>MALEEIRPKEVYLD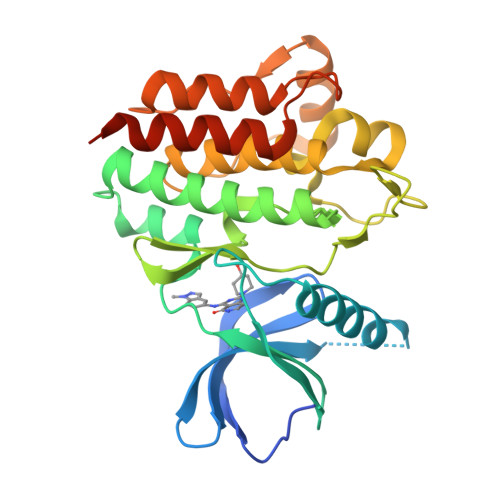RKLLTLEDKELGSGNFGTVKKGYYQMKKVVKTVAVKILKNEANDPALKDELLAEANVMQQLDNPYIVRMIGICEAESWMLVMEMAELGPLNKYLQQNRHVKDKNIIELVHQVSMGMKYLEESNFVHRDLAARNVLLVTQHYAKISDFGLSKALRADENYYKAQTHGKWPVKWYAPECINYYKFSSKSDVWSFGVLMWEAFSYGQKPYRGMKGSEVTAMLEKGERMGCPAGCPREMYDLMNLCWTYDVENRPGFAAVELRLRNYYYDVVNLEHHHHHHHH[2x]>MQRGSAYFLRGRARQNLKVLLLYCAFLLVMLLAYASIFRYLMWHLEGRAYSFMAGIYWTITVMTTLGFGDITFESDAGYLFASIVTVSGVIFLDIILPFGFVSMFLAPWIERRLRYHPTIELPDDTRGHILIFGIDPITRTLIRKLESRNHLFVVVTDNYDQALHLEEQEGFKVVYGSPTDAHVLAGLRVAAARSIIANLSDPDNANLCLTVRSLCQTPIIAVVKEPVHGELLRLAGANQVVPLTRILGRYLGIRATTCGALAHILDSFGNLQIAELPVHGTPFAGKTIGE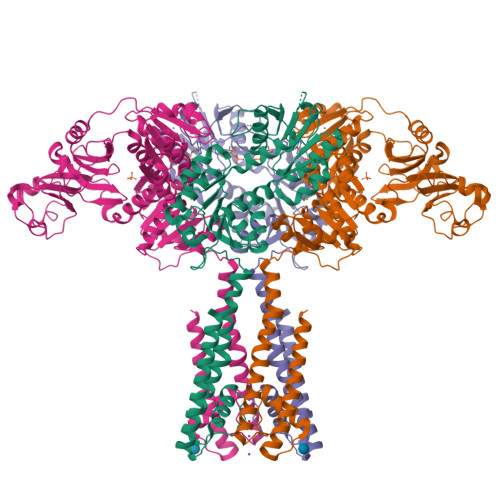SGIRQRTGLSIIGVWERGSLTTPQRETVLTEQSLLVLAGTKSQLAALEYLIGEAPEDELIFIIGHGRIGCAAAAFLDRKPVPFILIDRQESPVCNDHVVVYGDATVGQTLRQAGIDRASGIIVTTNDDSTNIFLTLACRHLHSHIRIVARANGEENVDQLYAAGADFVVSNASVGANILGNLLEHKESAFLSEGMAVFRRPLPPAMAGKTIAETRLRPLTGCSIVAIEAPDRADILISPPPETILAEGARLILIGTSEQEKTFDQTIAARLVPR[4x]> YSIEADKKFKYSVKLSDYPTLQDAASAAVDGLLIDRDYNFYGGETVDFGGKVLTIECKAKFIGDGNLIFTKLGKGSRIAGVFMESTTTPWVIKPWTDDNQWLTDAAAVVATLKQ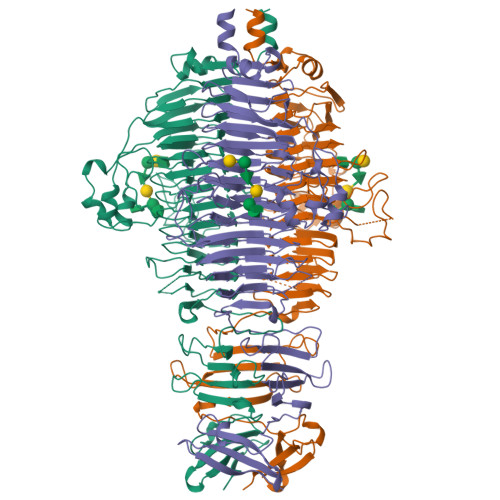SKTDGYQPTVSDYVKFPGIETLLPPNAKGQNITSTLEIRECIGVEVHRASGLMAGFLFRGCHFCKMVDANNPSGGKDGIITFENLSGDWGKGNYVIGGRTSYGSVSSAQFLRNNGGFERDGGVIGFTSYRAGESGVKTWQGTVGSTTSRNYNLQFRDSVVIYPVWDGFDLGADTDMNPELDRPGDYPITQYPLHQLPLNHLIDNLLVRGALGVGFGMDGKGMYVSNITVEDCAGSGAYLLTHESVFTNIAIIDTNTKDFQANQIYISGACRVNGLRLIGIRSTDGQGLTIDAPNSTVSGITGMVDPSRINVANLAEEGLGNIRANSFGYDSAAIKLRIHKLSKTLDSGALYSHINGGAGSGSAYTQLTAISGSTPDAVSLKVNHKDCRGAEIPFVPDIASDDFIKDSSCFLPYWENNSTSLKALVKKPNGELVRLTLATL SIMOCYCLINONE D8 | C46 H42 Cl N O18 | 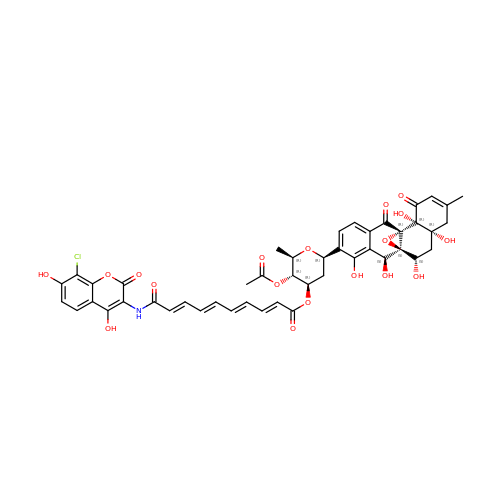PLEGMCYXNQPJNV-VHSVXIAXSA-N>LTPKETCDLCQIALRTVFGHFGGNIPSRRKLVHQLKHECKRHFNYRRRCLLLMKVNSDLIFREMTDGSFKPMEVCLIMRECNPHDSPLEPEMIDKS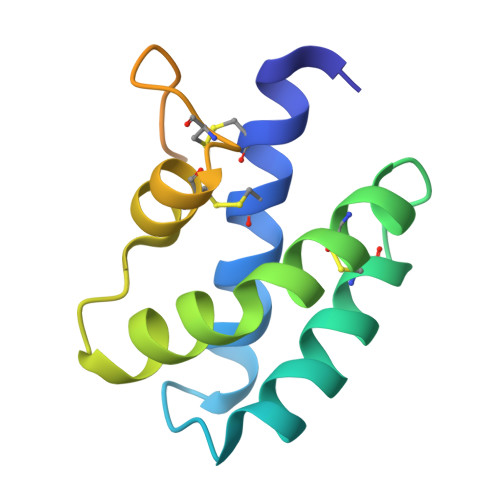GQPEAFALVSSSDDNYDTSEE[2x]>[3x]MVRIIVKNVSKVFKKGKVVALDNVNINIENGERFGILGPSGAGKTTFMRIIAGLDV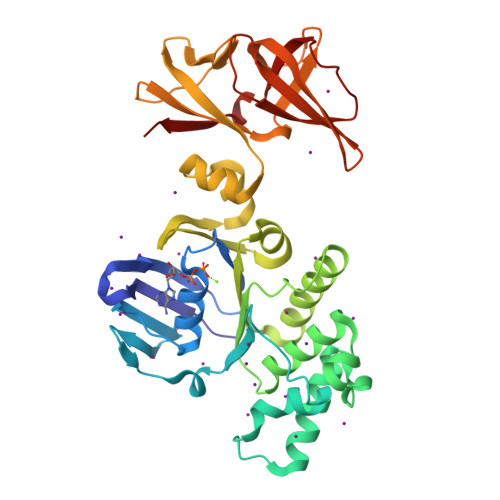PSTGELYFDDRLVASNGKLIVPPEDRKIGMVFQTWALYPNLTAFENIAFPLTNMKMSKEEIRKRVEEVAKILDIHHVLNHFPRELSGGQQQRVALARALVKDPSLLLLDEPFSNLDARMRDSARALVKEVQSRLGVTLLVVSHDPADIFAIADRVGVLVKGKLVQVGKPEDLYDNPVSIQVASLIGEINELEGKVTNEGVVIGSLRFPVSVSSDRAIIGIRPEDVKLSKDVIKDDSWILVGKGKVKVIGYQGGLFRITITPLDSEEEIFTYSDHPIHSGEEVLVYVRKDKIKVFEKN> GLIVDTRDVEERVHVMRKTKLAPTVAHGVFNPEFGPAALSNKDPRLNEGVVLDEVIFSKHKGDTKMSAEDKALFRRCAADYASRLHSVLGTANAPLSIYEAIKGVDGLDAMEPDTAPGLPWALQGKRRGALIDFENGTVGPEVEAALKLMEKREYKFACQTFLKDEIRPMEKVRAGKTRIVDVLPVEHILYTRMMIGRFCAQMHSNNGPQIGSAVGCNPDVDWQRFGTHFAQYRNVWDVDYSAFDANHCSDAMNIMFEEVFRTEFGFHPNAEWILKTLVNTEHAYENKRITVEGGMPSGCSATSIINTILNNIYVLYALRRHYEGVELDTYTMISYGDDIVVASDYDLDFEALKPHFKSLGQTITPADKSDKGFVLGHSITDVTFLKRHFHMDYGTGFYKPVMASKTLEAILSFARRGTIQEKLISVAGLAVHSGPDEYRRLFEPFQGLFEIPSYRSLYLRWVNAVCGDAAAALEHHHHHH

Replication of the FMDV genome is mediated by a viral RNA-dependent RNA polymerase (RdRp), named 3Dpol through a negative-sense RNA intermediate. RdRp uses VPg as a primer for both minus and plus strand RNA synthesis. The first step of the viral genome replication consists of the successive incorporation of two uridine-monophosphate residues to a highly conserved tyrosine residue (Tyr3) of VPg. This reaction, termed uridylylation, is also catalyzed by 3Dpol using as template a small stem-loop structure (cis-acting replication element (cre) or 3B-uridylylation site (bus)) that is located within the 5′-untranslated region.

Among them, 5-fluorouridine triphosphate (FUTP) is a potent competitive inhibitor of VPg uridylylation in vitro and also behaves as a potent mutagen for picornaviruses including FMDV. To gain insight into the role of FUMP-VPg1 in inhibition of further uridylylation, we co-crystallized 3Dpol in the presence of the modified 15-mer peptides FUMP-VPg1 and UMP-VPg1. Tetragonal crystals of the 3Dpol complexes were obtained in both cases. Analyses of the electron density maps showed that the VPg1 peptides could not be traced in any of the complexes, most likely due to disorder. However, best-fit structural superpositioning showed that 3Dpol crystallized in the presence of FUMP-VPg1 exhibited a large conformational change in the β9-α11 loop, located at the N-terminal motif B. On the contrary, the structure of 3Dpol in complex with UMP-VPg1 was practically identical to that of the apo form. Motif B is formed by a “loop-α-helix” structure located at the base of the template channel and is involved in ribonucleoside triphosphate (rNTP) recognition, template binding and translocation of the nascent dsRNA. In the apo form of 3Dpol, the β9-α11 loop is packed against the fingers domain, forming part of the template channel and participating in template binding. But in the presence of FUMP-VPg1, loop residues from Ser298 to Thr303 in this motif B appear displaced by 7.8 Å towards the active site, thereby closing the template channel and preventing the correct positioning of the nucleotide template in the active site pocket. Large movements of this loop have been observed ranging from an open conformation, in which the loop is packed against the fingers domain, leaving the active site cavity accessible for template entry, to a closed conformation where the loop is found inside the catalytic pocket, resulting in a conformation that sterically clashes with the template nucleotide. The structural data shown in this work, together with previous evidence of VPg fluorouridylylation, prompt us to speculate that the inhibitory effect of FU on VPg uridylylation might be explained by the stabilization of the β9-α11 loop in the closed conformation, thus preventing the correct positioning of the template nucleotide in the active site cavity of 3Dpol.> MRGSHHHHHHGRSLNPLSTPQFDSTDETPASYNLAVRRAAPAVVNVYNRGL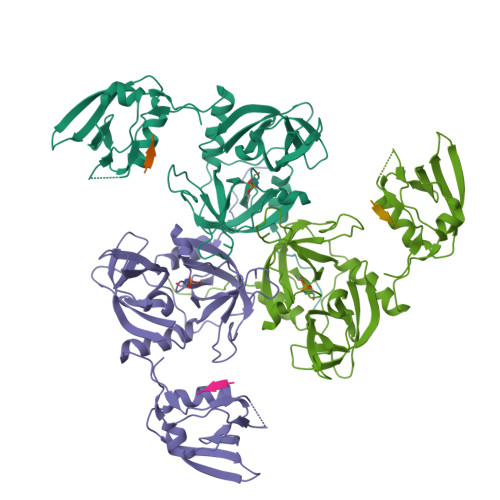NTNSHNQLEIRTLGSGVIMDQRGYIITNKHVINDADQIIVALQDGRVFEALLVGSDSLTDLAVLKINATGGLPTIPINARRVPHIGDVVLAIGNPYNLGQTITQGIISATGRIGLNPTGRQNFLQTDASINPGNSGGALVNSLGELMGINTLSFDKSNDGETPEGIGFAIPFQLATKIMDKLIRDGRVIRGYIGIGGREIAPLHAQGGGIDQLQGIVVNEVSPDGPAANAGIQVNDLIISVDNKPAISALETMAQVAEIRPGSVIPVVVMRDDKQLTLQVTIQEYPATN;> DNRDGNVYQF alpha-L-arabinopyranose | C5 H10 O5 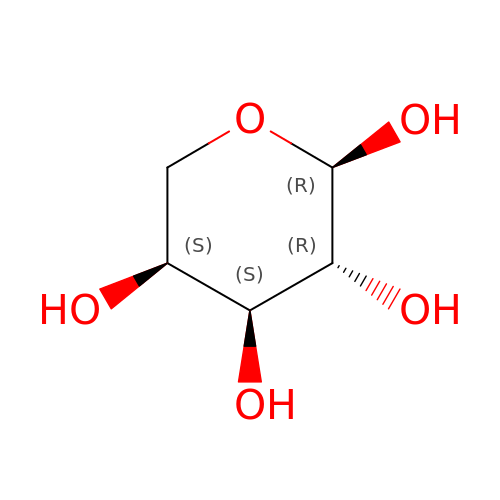| SRBFZHDQGSBBOR-QMKXCQHVSA-N>[4x]RDMPLDSDVFRVPPGYNAPQQVHITQGDLVGRAMIISWVTMDEPGSSAVRYWSEKNGRKRIAKGKMSTYRFFNYSSGFIHHTTIRKLKYNTKYYYEVGLRNTTRRFSFITPP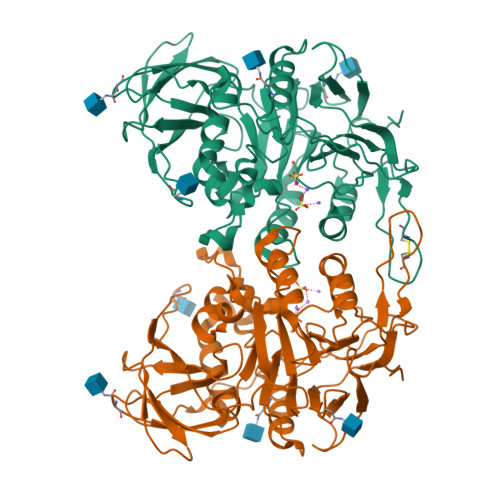QTGLDVPYTFGLIGDLGQSFDSNTTLSHYELSPKKGQTVLFVGDLSYADRYPNHDNVRWDTWGRFTERSVAYQPWIWTAGNHEIEFAPEINETEPFKPFSYRYHVPYEASQSTSPFWYSIKRASAHIIVLSSYSAYGRGTPQYTWLKKELRKVKRSETPWLIVLMHSPLYNSYNHHFMEGEAMRTKFEAWFVKYKVDVVFAGHVHAYERSERVSNIAYKITNGLCTPVKDQSAPVYITIGDAGNYGVIDSNMIQPQPEYSAFREASFGHGMFDIKNRTHAHFSWNRNQDGVAVEADSVWFFNRHWYPVDDST>GGMGQTLLDALNVRVVGSGERVLVL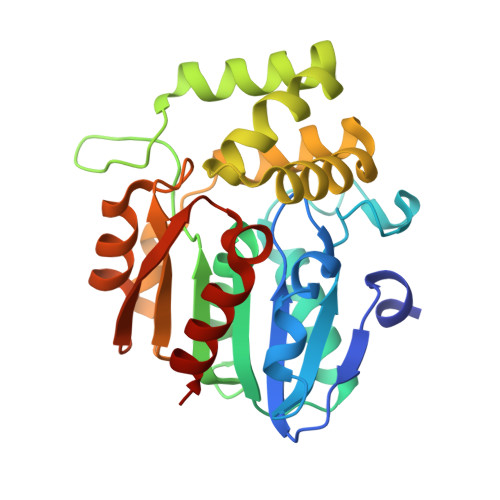AHGFGTDQSAWNRILPFFLRDYRVVLYDLVCAGSVNPDFFDFRRYTTLDPYVDDLLHILDALGIDCCAYVGHAVSAMIGILASIRRPELFSKLILIGASPRFLNDEDYHGGFEQGEIEKVFSAMEANYEAWVNGFAPLAVGADVPAAVREFSRTLFNMRPDITLFVSRTVFNSDMRGVLGLVKVPCHIFQTARDHSVPASVATYLKNHLGGKNTVHWLNIEGHLPHLSAPTLLAQELRRALSHR[12x]2-[3-(aminomethyl)-4-(2,4-dichlorophenyl)-2-methyl-5-oxo-5,7-dihydro-6H-pyrrolo[3,4-b]pyridin-6-yl]-N,N-dimethylacetamide 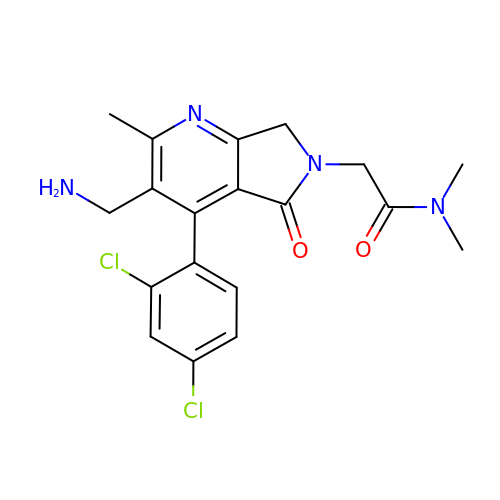| C19 H20 Cl2 N4 O2 | PECDPZCIECMGCM-UHFFFAOYSA-N>MRGSHHHHHHGSACELSSKHDYTNPPWNAKVPVQRAMQWMPISQKAGAAWGVDPQLITAIIAIESGGNPNAVSKSNAIGLMQLKASTSGR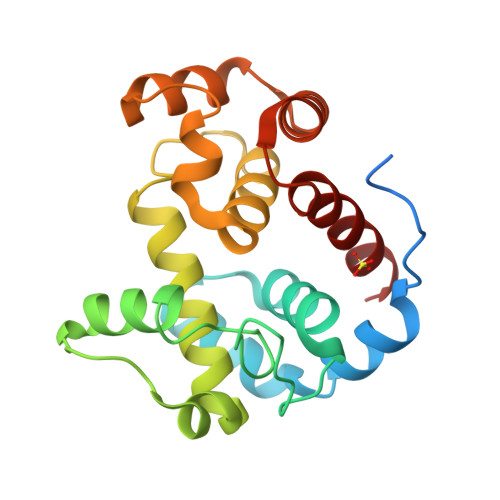DVYRRMGWSGEPTTSELKNPERNISMGAAYLNILETGPLAGIEDPKVLQYALVVSYANGAGALLRTFSSDRKKAISKINDLDADEFLEHVARNHPAPQAPRYIYKLEQALDAM[5x]>QDEVLSEAFRLTITRKDIQTLNHLNWLNDEIINFYMNMLMERSKEKGLPSVHAFNTFFFTKLKTAGYQAVKRWTKKVDVFSVDILLVPIHLGVHWCLAVVDFRKKNITYYDSMGGIN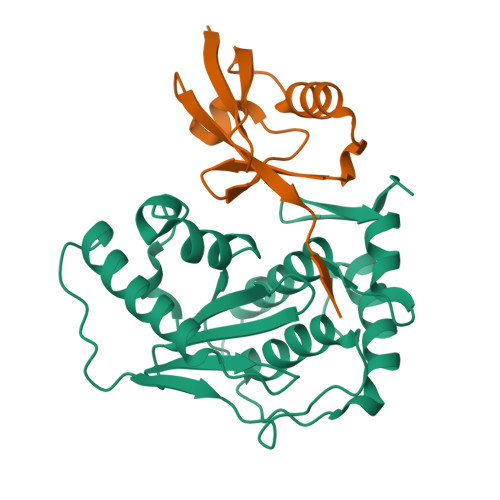NEACRILLQYLKQESIDKKRKEFDTNGWQLFSKKSQEIPQQMNGSDSGMFACKYADCITKDRPINFTQQHMPYFRKRMVWEILHRKLL[2x];>[2x]EYIKLKVIGQDSSEIHFKVKMTTHLKKLKESYCQRQGVPMNSLRFLFEGQRIADNHTPKELGMEEEDVIEVYQEQTGG>[2x]GMDLSRINTWKSKQ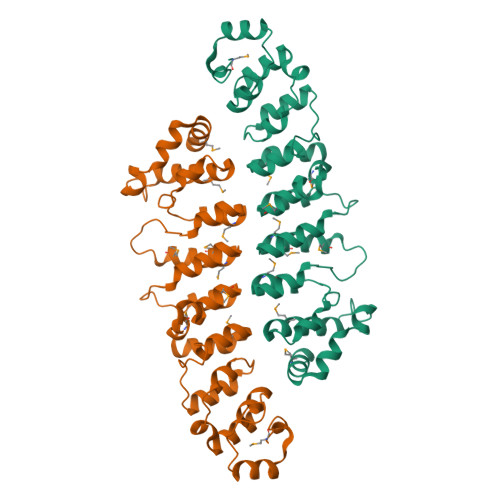LKSFLSSKDTFKADVHGHSASYYAIADNNVRLVCTLLNAGALKNLLENEFPLHQAATLEDTKIVKILLFSGLDDSQFDDKGNTALYYAVDSGNMQTVKLFVKKNWRLMFYGKTGWKTSFYHAVMLNDVSIVSYFLSEIPSTFDLAILLSCIHITIKNGHVDMMILLLDYMTSTNTNNSLLFIPDIKLAIDNKDIEMLQALFKYDINIYSANLENVLLDDAEIAKMIIEKHVEYKSDSYTKDLDIVKNNKLDEIISKNKELRLMYVNCVKKN> MQNSQTFSVTELSLPKGGGAITGMGEALTPAGPDGMAALSLPLPISAGRGYAPSLTLNYNSGTGNSPFGLGWDCGVMAIRRRTSTGVPNYDETDTFLGPEGEVLVVALNEAGQADIRSESSLQGINLGATFTVTCYRSRLESHFNRLEYWQPQTTGATDFWLIYSPDGQVHLLGKNPQARISNPLNVNQTAQWLLEASISSHSEQIYYQYRAEDEAGCETDELAAHPSATVQRYLQTVHYGNLTASDVFPTLNGDDPLKSGWMFCLVFDYGERKNSLSEMPLFKATGNWLCRKDRFSRYEYGFELRTRRLCRQILMFHRLQTLSGQAKGDDEPALVSRLILDYDENAMVSTLVSVRRVGHEDNNTVTALPPLELAYQPFEPEQTALWQSMDVLANFNTIQRWQLLDLKGEGVPGILYQDRNGWWYRSAQRQAGEEMNAVTWGKMQLLPITPAVQDNASLMDINGDGQLDWVITGPGLRGYHSQHPDGSWTRFTPLHALPIEYSHPRAQLADLMGAGLSDLVLIGPKSVRLYVNNRDGFTEGRDVVQSGDITLPLPGADARKLVAFSDVLGSGQAHLVEVSATQVTCWPNLGHGRFGQPIVLPGFSQSAASFNPDRVHLADLDGSGPADLIYVHADRLDIFSNESGNGFAKPFTLSFPDGLRFDDTCQLQVADVQGLGVVSLILSVPHMAPHHWRCDLTNAKPWLLSETNNNMGANHTLHYRSSVQFWLDEKAAALATGQTPVCYLPFPVHTLWQTETEDEISGNKLVTTLRYAHGAWDGREREFRGFGYVEQTDSHQLAQGNAPERTPPALTKSWYATGLPAVDNALSAGYWRGDKQAFAGFTPRFTLWKEGKDVPLTPEDDHNLYWLNRALKGQPLRSELYGLDGSAQQQIPYTVTESRPQVRQLQDGATVSPVLWASVVESRSYHYERIISDPQCNQDITLSSDLFGQPLKQVSVQYPRRNKPTTNPYPDTLPDTLFASSYDDQQQLLRLTCRQSSWHHLIGNELRVLGLPDGTRSDAFTYDAKQVPVDGLNLETLCAENSLIADDKPREYLNQQRTFYTDGKNQTPLKTPTRQALIAFTETAVLTESLLSAFDGGITPDELPGILTQAGYQQEPYLFPRTGENKVWVARQGYTDYGTEAQFWRPVAQRNSLLTGKMTLKWDTHYCVITQTQDAAGLTVSANYDWRFLTPTQLTDINDNVHLITLDALGRPVTQRFWGIESGVATGYSSSEEKPFSPPNDIDTAINLTGPLPVAQCLVYAPDSWMPLFSQETFNTLTQEEQETLRDSRIITEDWRICALTRRRWLQSQKISTPLVKLLTNSIGLPPHNLTLTTDRYDRDSEQQIRQQVAFSDGFGRLLQASVRHEAGEAWQRNQDGSLVTKVENTKTRWAVTGRTEYDNKGQTIRTYQPYFLNDWRYVSDDSARKEAYADTHIYDPIGREIRVI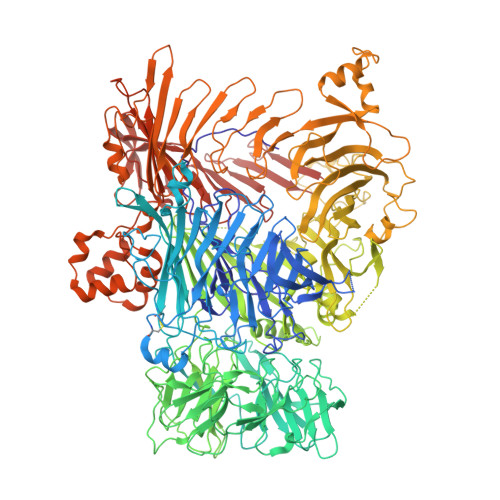TAKGWLRQSQYFPWFTVSEDENDTAADALV> MVSGGVVQLISYGAQDVYISGGPKTIFKSYVKKVNNFAIDSVKIPINGMGNGNPSVLIPRNGDLIKSIRLEITLKKGTGQSFYPAEQLISYLALKIGGNIIQKIDDFSNFCRIRNELFMDPD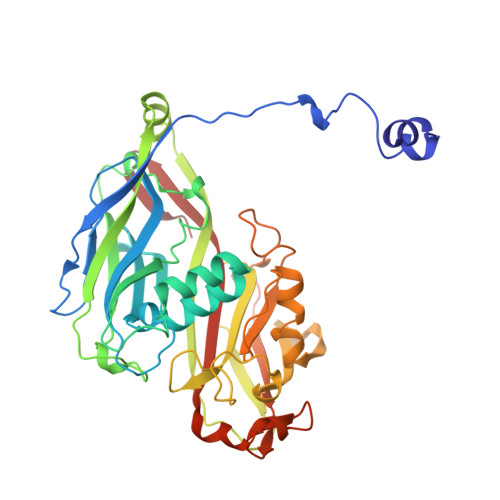ERHTDYRVNNFSSSDVVGSVKYFFLDLPLFFSKDTSVALPLIALQYHDIELDFRFNDVSTIQGVDASYTPTIEMYIDYVYLEQQERIKLVEKPLFYNIEQCNFYRKDITFPALSSTFKLDIPFNNPSRFLVWYFNTDSFGIYNTSGLYFNSNDAAAPLESAVMLLNGTERFKSREGMYFNCVQPQQALGRSPSSGIYMYAFGEDVANATSKGALDMSRVNELSLQLTTKNATAANVYTVYNPQETLASSTSTYKGITLFSTNWNVLQVRSGLGAVMFDS> MQNWTLVWQDEFTNGISSDWVFETGNGNSGWGNNELQYYRRENATVENGNLVITAKR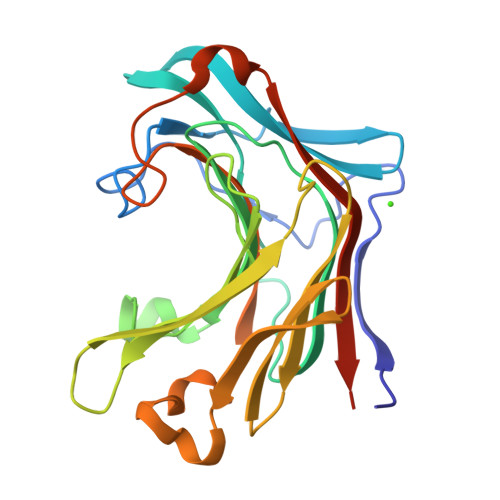ESIGGYNYTSTRMKTQGRKSWKYGKVEARIAMPSFMGSWPAFWMLGDNISSVGWPACGEIDIMEHVNTEAQTHGTIHWQDHNNTYANYSGSIPVSSVTSYHIYTIEWDASVIKWFVDGNLYHEASIANGVNGTSEFHNNFFILLNMAIGGNWPGFNIDNNAFPARMLVDYVRVYQKTDLEHHHHHH> MGSSHHHHHHSQDPSSMTMELRPSGDSGSSDVDAEISDGFSPLDTSHRD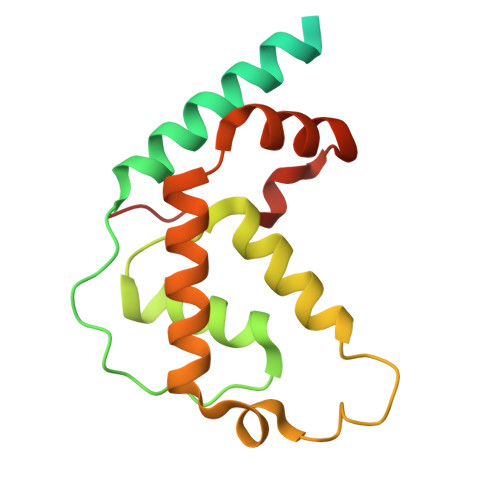VADEGSLLRRAEMYQDYMKQVPIPTNRGSLIPFTSWVGLSISMKQLYGQPLHYLTNVLLQRWDQSRFGTDSEEQRLDSIIHPTKAEATIWLVEEIHRLTPSHLHMALLWRSDPMYHSFIDPIFPEK> GAACGACATTGA;> CGAGGACTC;> TCATCG;>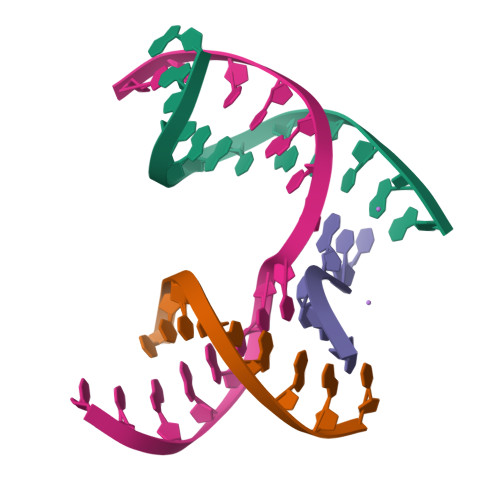 TCGAGTCCATGTCGT(Z)-OCTADEC-11-ENYL 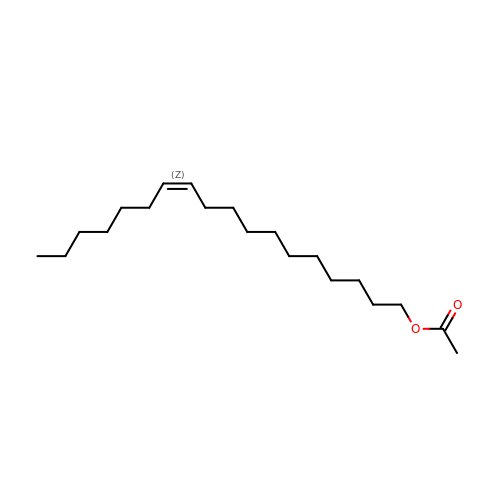ACETATE | C20 H38 O2 | QSZKEDWVAOAFQY-HJWRWDBZSA-N>MAHHHHHHSSGLEVLFQGPMTHSVVELIEIESAIIQVKMQDRTHKNAFSQELTDDLIQAFEYIRQNPKYKAVILTGYDNYFASGGTQEGLLRIQQGLTKFTDDNLYSLALDCEIPVIAAMQGHGIGGGFVMGLFADIVILSRESVYTANFMKYGFTPGMGATFIVPKKLGFSLAQEILLNAGSYRGADLEKRGVPFKVLPRAEVLDYAVELAQELAEKPRNSLVTLKDHLVAPLRDQLPRVIEQELMMHEKTFHHEEVKSRIKGLYGN[3x]

In this study we present a structural and functional description of the bacillaene synthase β-branching enzymes PksH and PksI. These biocatalysts are responsible for the final two steps in β-methyl branch incorporation in this PKS/NRPS pathway. There is a single active site per PksI monomer, with each active site positioned on the periphery of the trimer, ~ 43 Å from one other. Akin to PksH, PksI adopts a characteristic CS fold, with a ββα core, that comprises two approximately perpendicular -sheets surrounded by -helices.

Two crystal structures of PksI were elucidated; the first to 1.93 Å resolution using a crystal cryoprotected in glycerol (PksI_GOL), and the second to 2.1 Å using a crystal cryoprotected using ethylene glycol (PksI_EG). The final model of PksI_GOL comprises residues 1–247 of chain A, residues 4–249 of chain B and residues 3–231 of chain C, 663 water molecules, 6 glycerol molecules and 1 HEPES molecule. In the PksI_GOL structure a single monomer (chain A) within the PksI trimer possess a bound glycerol molecule within its active site. Comparison of the active site architecture of PksI monomers in glycerol bound and free states allows assessment of active site reorganization as a consequence of ligand binding. In the unliganded structure, the active site adopts an “closed” conformation, with the side chains of Phe136 and Phe81 pointing directly into the centre of the active site cavity and His230 rotated to face away from the central chamber. In the liganded structure, the active site is occupied by the substrate mimic glycerol, whose hydroxyl group can form a hydrogen bond with His230. In this “open” conformation the side chains of Phe136 and Phe81 are seen to flip away from the centre of the active site, which is occupied by the bound glycerol molecule. As a consequence, Phe136 forms a tripartite stacking interaction with Phe234 and His235, which sits beneath the proposed catalytic residue His230, which itself rotates to point directly into the centre of the active site. It is likely that our unliganded structure represents the ground state of the enzyme, with the glycerol bound form equating to a mimic of a PksI reaction intermediate. The observed side chain rearrangements in the glycerol bound structure are essential for allowing the substrate to be accommodated within the catalytic site of the enzyme and may also function to promote active site solvation, consistent with a potential role for water as a proton donor during catalysis.> AEYVRALFDFNGNDEEDLPFKKGDILRIRDKPEE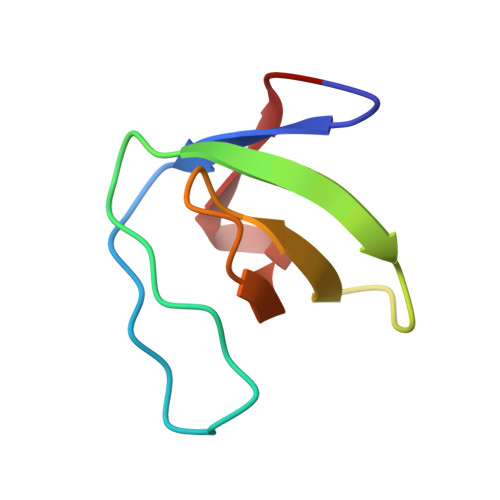QWWNAEDSEGKRGMIPVPYVEKY>[3x]MEATLITQPHATGHVGNFFFTHWKDGGSAALDLDAKGNFSVSWQGG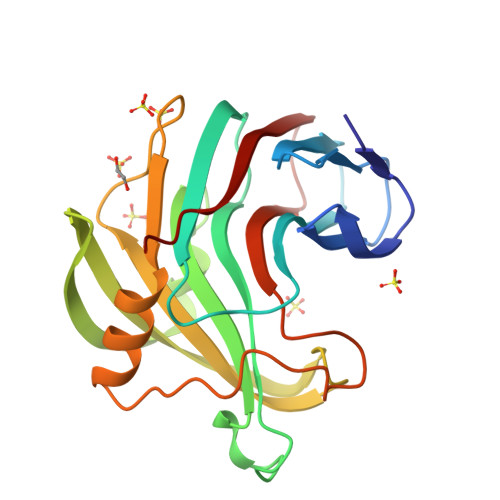GYNYVGGPGWHFGDKNRVIGYRFNQDSGASYITLYGWGYDKSMPATDPAHLVEYYILQRWTYDPSQDGIYGKTFVSNGIEYSTYRSIRKVKPSINGPTTFYQYWSKPSAQQELGKDHKIIFADHVKAWADTGWILPDMNNFDASDDPTYQVLAVEVFNPQKNGTASGQVWDETPR> NV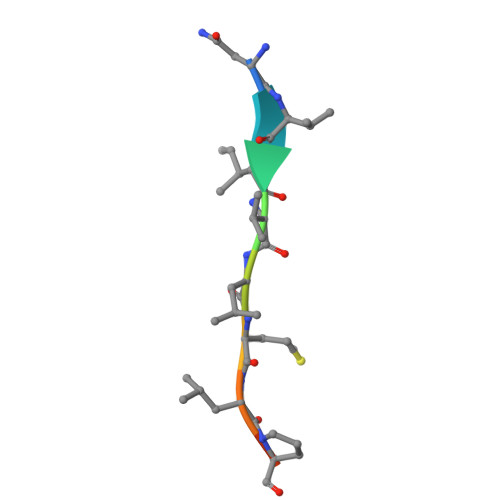IVLMLPME>MGSSHHHHHHSQDLENLYFQGGSTRLSLEAMLAERAMVARQDLAGLKRKLAGADRVLAPQSPEQCGRESAQAQARSVTSELKSAVKEAQGLEHQTLDFLEQLGEYPVCGILHGDHPVHPSGTHNNNGKVSVKRQFAAGVNTSDALTCAFRFEDSDLVRETALKTTYTDGTWAGFVQRLKMQTTRKCVQEKVSRKLLKQLFPYDPQKLVDVSGELSELVLGIKTNAIASAGPPYWRTKRDALPDMLDCVLPLLYDHIVRKDLTTLRNKHPELFLAECKNKTDRYEVESLGEKTRPYFSHPFHLSALVSVLSQSFSGALKIMTEDSTSFNAYGFSWTNGGAEDLAIWARQAGEAGKKPPRIACYGDDTDIYYRKDGKLYRICPDFKQMDGSVDATTIEAVVDYVVDAHVKQYPTARQFWEEVGKLWVEMATQSPFLIDGTKVYRKMQKDGLMTGVVGTTLFDTVKSALAYNDWADQLMFGSLNLLEEKYAIEFFKNKHGLVIKEGTWKPALVNEDPGFGELWTEQKFLGLQLKVV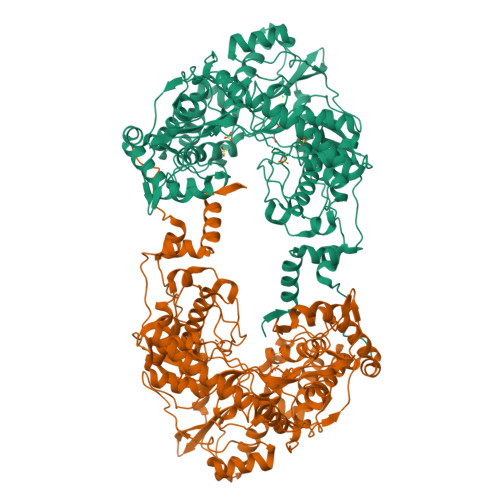RRENEKVYVPNLPFEDWLTMWVTPRSKYRSKETETMRERTLFDRARGLLVTGAVFDERARGLMGAVINSTAPEVVCMRVQEGGGRGAPPAYAFLTRDGVFEFPISDGYPSYDWVVSLYSRDHPCDMPRVFPEAATLIASYRKQVMDTRVVI[2x]>MRRFGSKFASGLASRCALACPLASAATAPAGASTTSSTSSAQKSFFKTTEMIGYVHSIDGTIATLIPAPGNPGVAYNTIIQIQVSPTTFAAGLVFNLEKDGRIGIILMDNITEVQSGQKVMATGQLLHIPVGAGVLGKVVNPLGHEVPVGLVTRSRRLLDSTLGKVDTGAPNIVSRSPVNYNLLTGFKAVDTMIPIGRGQRELIVGDRQTGKTSIAVSTIINQVRINQQILSKNAVISIYVSIGQRCSNVARIHRLLQSYGALRYTTVMAATAAEPAGLQYLAPYAGVTMGEYFMNRGRHCLCVYDDLSKQAVAYRQISLLLRRPPGREAYPGDVFYLHSRLLERAAMLSPGKGGGSVTALPIVETLSNDVTAYIVTNVISITDGQIYLDTKLFTGGQRPAVNIGLSVSRVGSSAQNAAMKGVAGKLKGILAEYRKLAADSVGGQQVQTIPMIRGARFVALFNQKQPSYFMNAIVSLYACLNGYLDDVKVQYVKFYEYLLVHRDLGIMYGTAKNKFFYMYVQELNYLIRFFTLNSPILHGELEEMLKQHTHLFLQHYQSKMNAIKSEKDVKALKNLLYSCKRAV[3x];>[3x]MLTRFRSAVLRGAVSITGARAASTAPVADHKGRVGHVSQVIGAVVDVHFADGVPPVLTALDVVDKLGRDEPLTLEIVQHLDAHTGRCIAMQTTDLLKLKAKVVSTGGNISVPVGRETLGRIFNVLGDAIDQRGPVGEKLRMPIHAVAPKLADQAAEDAVLTTGIKVIDLILPYCKGGKIGLFGGAGVGKTVIIMELINNVAKGHGGFSVFAGVGERTREGTDLYLEMMQSKVIDLKGESKCVLVYGQMNEPPGARARVAQSALTMAEYFRDVEGQDVLLFIDNIFRFTQANSEVSALLGRIPAAVGYQPTLAEDLGQLQERITSTTKGSITSVQAVYVPADDITDPAPATTFSHLDATTVLDRAVAESGIYPAVNPLECASRIMDPDVISVDHYNVAQDVVQMLTKYRELQDIIAVLGIDELSEEDKLIVDRARKLVKFLSQPFQVAEVFTGMTGHYVQLDDTIDSFSGLLMGTYDQVPEMAFYMVGGINSVLEKAKKMAEEAAELEKMRRARVAQASS;> MSGKLRLYKEKLEGYNRFYSIVKTIKMVTLAKYRAAQGRIRTRDFSLRYTELAFSKPQASRDAVVAAKNALVYIPITTNRGSCGALNSNIVRCIDSVVSSKMVLMPVGKRGIDSFSKLYPDEFRYGIINDMKESMHFGYATFVIENAYEVSKDADRYQVIFNRFVSAGVQRNAVYNIPSYEKWKEDLADAASSDNQKNRYLFANALQNEEEQLIRDFFDFHAALAVLNAVGENELSEQAARLVAVEGQLTNISSLQQRTSSLYNKTRQFGITAALIEILSAMSSLEGNAMKGVRRNKFWEGAVTK;> MFRTFGRRLVSCTLPLLQSAPHDLPEGFEFMEHKVVNKDIHAPHENLETLRLTLTRQDEFLLREEPVKCVTVTGTNGEYGIYPGHAYKIVQLNPSPLTVEYTDGTTKKYFVSGGFAHINNEGSCDVNTVECTLLDDLDLAIAEKELAAQQAALGSAKDDKAKSVVEIRISVIEAVIAALKHH;> MIRRSCALLSSSWRDHGISYLKYLNVCTETLHSTVKESRRAKYERWSKPCYTAQRPDGAGGQETIDKVPIHTKDY;>[3x]MMRRVYSPVFCSVAAARFAATSAAKKYDLFGYEVDTNTAPWIEKIKKCKYYDEAGEVLVNMNVSNCPPDIATYNATLQCIYQSPSKQSTPVDNESKFCAMMDLLEEMQHRNRLKPNEESWTWVMKECVKSGQFRLGYCIQQVMETECKGCPADLVKANEANAQKAKTEGKEHPGHLSQQAGLFDVKVE;>MSAKAAPKTLHQVRNVAYFFAAWLGVQKGYIEKSANDRLWVEHQRKVRQQNVERQQALDSIKLMQQGVRATTPGQLEGVPAELQQLAEAFTK[2x];>[2x]MSSTKCAVACKIMTPLCNAASKVQARSAKKLAALTDAGIQKTISEHNANGTDAAVSSTKRYLAEQRQLFHYRVVRFFDECHYIISGEYFAQYTKVNLIWDLRFLTKLVVLFLIGTVLGRQSIFPPIDPDSPLVEALVTKVNPNY;> MFRRLSSSARAVVAARFYTPPEGLKKLYASDFENSKYPLNIVPSDSVLFAKFLYKAAEEKGNFDNILSDFQKIAAAASKLPIFWERTAVVEKIPEFKQLSEPTFFTLVWMQNNGMLELIQEVAEVYETFVNAKQKKAVAKIFVAPGGEKNVEEARRVAEELHKGLKELADYTLVLKTVVDRTIVKGFAVELAGQYVNKAEGQQKQAGRADEVDYTNLPAPKPQKTVWDDNIETEVLRKYLDGLSQYDMEEAKYGV;>[10x]MMRRLALQSSIRRATPFATPLVASTKALNPMCSAITIREASTVAISVQGLHYVGTGLAAIALAGVGLGIGTIFGNLLVACARQPNLTKMLFNYAILGFALTEAIGLFALMLAFLMLFS;> MFLFFFCDLFWLRLLLCMYYCVWSRLCFIVYFNCLMLIFDFLLFCLFDLYLFVGLCLFLLLWFMLFNLYSLILYYCITYLNLYLLFCIVFLLYIAFLFLFCFLCDFFLFNNLLVGDSFMDVFFIRFLLCFLECFSLLCRCLSTFLRLFCNLLSSHFLLLMFFDFFYFIFVFFFYGVFCYWFILFIFVFCFCLLFYVFLYLLDLFAAILQLFIFCNMILQLIMDFLLFLLFV;> MLRRLGANVSNMARPMNKYAVTVSPRRHLEPMSTWYLASWAMVWYYAFFFWMPMVWTDIMVPSFVYNKLPVIHFLQEKRAEQKLRRVLDETYTEWTEELDQAHVTDAITRSLNI;> MRRVSSPNIT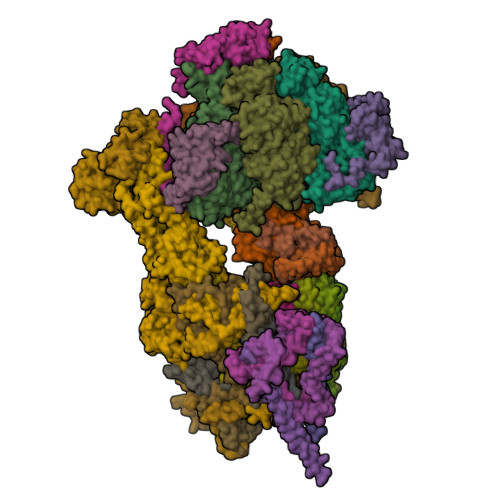IQSVRWISGVSPLLYFPPTTTSTTNREDQINKNTNIAIQMIKRYKGEVPPHYTRKSSATIEQVEKEIDALLGGAEKLRKTSTDDQPMDKLTLMERCLRHALWSYHKEEGRYDFDQIGRWVVYTPEDEVKLAQLKREVEAKEKLAALRKRREEEGLPGGPVPRINWPQEYSSFIDREPVVAKRIRYDTLASTTLERDEKQIESTLQQYRRASQDKRLDDLVDLLERFKPVLAREAIMQRLTIKHLEGQLGVWRYMDWCPEVRDRAELEVDITGWQWWSPLEERRLLPVRLRSVNEVREIMSKTQAKKSAEAAERNPIVTQTSTGDNARDRLLKEVLALQARINQRDEVEPSQTEQKKKAHH;> MQGSWSVLKKNCSNFFPGLLAFAQQTQEAYGIWLRIYNRQQKYGPTDFVEQSETFSPDYHKRFHSQDKNMWVDKELCTEVSQKEVARLMTYKLDMWRMAHCAGALLATGGYAIPFGLFWLANDTWVPSSFNLTGEELRAWREAQDLYRYRSAPSYLTDTKWHFDFHAYPWNETQERAWDDLFEKNDVRRDPKVVRPAAEMYDGFIKFELIRRKSLRHLCRSMNIPTFPMLARLCNGTRVRDYWNLAWCEDYMVITQRLHESMTDEELYDYAWRRYLAPYDKNLNREQLMERVEDYFEFLGPDFVAHGKAPNLVILTNYVLGYYNDPAYLEGDISELDKNDYDHLASWGKDAFLRRLEFENGPLRDQVEAHTQRLLAERAAIAKGDNAAAVEGRHTA;> MVLFSTYRSSRLVSKEFLHGPVMRFRALGEYYFQRAWNGTLNWALPGEYRLYAVMIPFIYFYHRWHNDHTLDRDHVEKAMIMRWGGTLEDVRKLSAKDQLRVRCFTDIEKLYSAYGPKDTYLQPPGDTLPGKDFYRKAGGAQAHH;> MSKQLTFISAGATAAVLQSASAIVSKVAGGRVQTKTAKEAGRHAVVVGPETPIGVHTAVTEVPKSAQDPLFSGVSTVVVRAVLPRAAPDSVQLRDALDVYASAGIDTKEEVRSATEAFKKSAEVAVGKAKAKGVKRIVLVVKQASKHNCINELFKKISTETIESAGLTTEVVGTAAVANQLIVNPESLGVVLLNDVAATEQIELAFAGVVGGVSRVYHTVEGGKISAGHSFKSVALAVAQELRELGLSSEADKVEAAASKNPRAVVSAL;> MRRTFISFSAASAAAAAPVTSTKMQTLHKLLTGEVSFKNKAPVKDCNIVHQFGENWATELSAYAKTLPAEQQKIIVRQIARVKLTRYTVAELAAYCGDGPALLDETARAANIEQGVAFVKAKGVEAFEKYVAEESTNANWKPEEAKKFIEDVKAKAK;> MVYTRWKCDRLPVFQLKLFTQEYPMHAAVGIFTIIFLWKHMSHCSEETERKYGWWAGYPYWRDPIARRNETKYKQMIINNDVDITHPKWTGCSVEQLEELSRVV;> MTKYELKMQYFDEWMIRWRKFQTESDWEIEKGRQWWRRFNMAVSGALFCGLVLYTSGTATLKRQYGLPHFFDIGVDGQAKETMLKTLTSRWRYTPQGYGRVLITGVPTYILFVTLEHYRERRRMQQYLQQNTVFGEQMRRLLSTGKIEEYLPVNIKATLPASQQAIYNY;> MLRRSSAALIRRTPVRHSGGELFVRPKLEEIPPADQCRGFFGPLNDSLKFLRLLDIKWMMNRAVAMRREYLIATPTLFTFIWMFTWKGAVIYFWGDRAPPRRMDWNTEETGRLPLGFKPTPAPL;> MLRKTPLFAMATTRKALVGNGPTFSTGGECMNTCDIQNAFPMNDRGVRSSSPFQEPNTAIYDSYLAWTYFQPMDVHIEKLPAPEAKYYQRHTKKPWDVSSTELTEIQSRKKYFQTLGYLVAFIYLYFLMPKEKSFSGLSGPDGHWIMLPKGRPELF;> MSSGFHFHDVSNDAIKGMPPSEALHKHLENAQLAHRICLAKALKAGEPPVEKCALTWGEVLIRYQAWSEYRPPFQDSVAQAKYKKYWSKKRQEEDDKNPFK;> MLRRLVPRVMMAPMGGATALCTSRGYNMLVFRDPKRRPQLSEEERAKVVVNQAEWPEEFKDFDPDDPYKNSPEIIKGMSSWNLFLWGVECAFIYQFYELVFPKSI;> MTENIEAVMSDFWSNPADHFRPNLKALTLYAERQHYVDRWLHVKERWLAPWYLPWWSPLFQLGTWYSQRSRNLFLVENHLSYRPYKFRRNDEDRNNPY;> MLLGGFVPRRFSQFNRDPCWMFFIFSVGFWLGEYPAMMIKYNARDLVYDPHRYVWSHHDDHH We later discovered that H. pylori encodes an atypical species‐specific bifunctional dehydrogenase/isomerase enzyme FabX, which introduces a cis‐double bond to the saturated acyl substrate of ACP via a backtracking mechanism that expectedly reverses the conventional fatty acid elongation direction. FabX utilizes a nitronate monooxygenase (NMO) flavoprotein family conserved flavin mononucleotide (FMN) cofactor and an active residue His182 inside the catalytic tunnel to extract electrons/protons from the acyl substrate for dehydrogenation and cis‐double bond formation, storing the captured electrons in FMN and [4Fe‐4S] cluster cofactors, respectively. Subsequently, FabX transfers the stored electrons back to the oxygen molecule located in the oxyanion hole between FMN and His182, generating superoxide (ROS), which is further excreted by H. pylori as a major source of peroxide, likely enabling its pathogenic function of gastric mucosa corrosion. Here, it is demonstrated that FabX is essential for H. pylori growth and gastric colonization by retaining UFA synthesis and producing ROS, respectively, and is a species‐specific anti‐H. pylori drug target.

Notably, compound 8j (annotated as FBX‐1872, hereinafter) exhibited potent FabX inhibition but only low antibacterial activity with a minimum inhibitory concentration (MIC) value higher than 64 µg mL−1. This could be due to the fact that the carboxyl group of 8j readily deprotonates and acquires negative charge at physiological pH, which reduces its lipophilicity and prevents it from permeating the bacterial cell membrane. Given that FBX‐1991 exhibits moderate solubility, we employed its highly similar analog, compound 8j (FBX‐1872), for further evaluation of binding affinity evaluation against FabX. FBX‐1872 exhibits comparable inhibitory activity against FabX as FBX‐1991 (IC 50: 0.437 ± 0.042 × 10−6 m) and increases the stability of FabX by ≈20.8 °C (ΔTm) at a concentration of 50 × 10−6 m. As expected, FBX‐1872 binds to FabX with a K d value of 0.435 ± 0.046 × 10−6 m. In addition, we also determined the crystal structure of FabX in complex with FBX‐1872 in space group P21 at a resolution of 1.60 Å. The structural comparison suggested that the structures of FabX–FBX‐1991 and FabX–FBX‐1872 complexes are highly similar with an RMSD value of 1.919 and both inhibitors adopt exactly the same conformations inside the catalytic tunnel of FabX, indicating similar inhibitory mechanisms of these inhibitors.

> EHHHHHHHMVSTLKPLKIGKHTIKFPIFQGGMGVGISWDELAGNVAKEGALGVISAVGTGYYKNMRFVERIVAKKPFEALNFYSKKALNEIFANARKICGNNPLGANILYAINDYGRVLRDSCEAGANIIITGAGLPTNMPEFAKDFSDVALIPIISSAKALKILCKRWSDRYKRIPDAFIVEGPLSGGHQGFKYEDCFKEEFRLENLVPKVVEASKEWGNIPIIAAGGIWDRKDIDTMLSLGASGVQMATRFLGTKECDAKVYADLLPTLKKEDILLIKSPVGYPARAINTGVIKRIEEGNAPKIACVSNCVAPCNRGEEAKKVGYCIADGLGRSYLGNREEGLYFTGANGYRVDKIISVHELIKELTEG> MSTIPSEIINWTILNEIISMDDDDSDFSKGLIIQFIDQAQTTFAQMQRQLDGEKNLTELDNLGHFLKQSSAALGLQRIAWVCERIQNLGRKMEHFFPNKTELVNTLSDKSIINGINIDEDDEEIKIQVDDKDENSIYLILIAKALNQSRLEFKLAR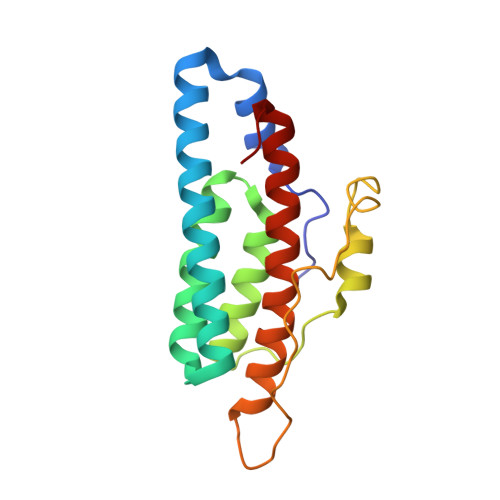IELSKYYNTNL>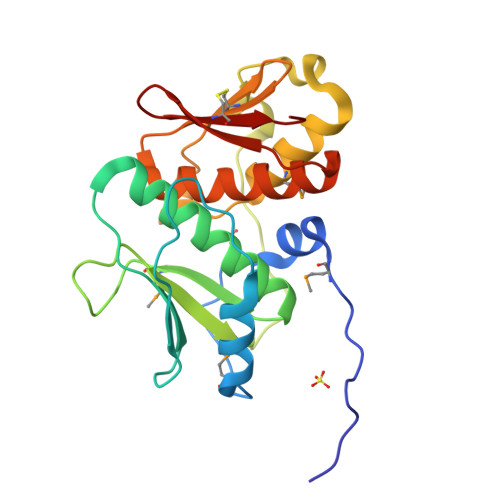 MGSDKIHHHHHHMNIFEAIENRHSVRDFLERKMPERVKDDIENLLVKFITKKLDWKINLSSFPSYIYAKAEKHFDELVEYGFQGEQIVLFLTAQGFGTCWMARSPHPDVPYIIVFGYPRTRNFTRKRRPITSFLENDLEELPPEIVKIVEMTILAPSALNRQPWKIKYTGGELCISSERPVDLGIALSHAYLTAREIFKREPVIQKRGEDTYCLILNP> DSDIKPLRMDPPVYPRMAQARGIEGRVKVLFTI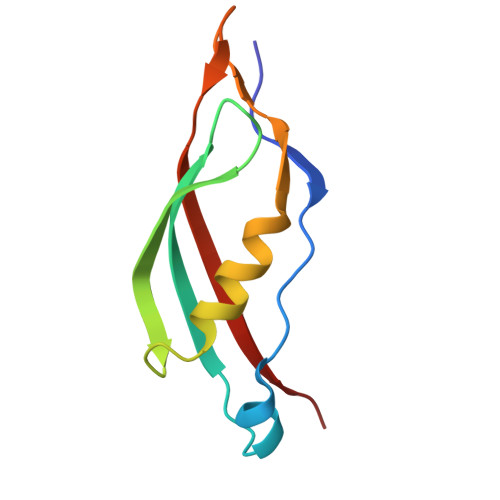TSDGRIDDIQVLESVPSRMFDREVRQAMAKWRFEPRVSGGKIVARQATKMFFFKIEK>[6x]KNKLYKNIEIDTDTHSVYIHSENKKILLNLTL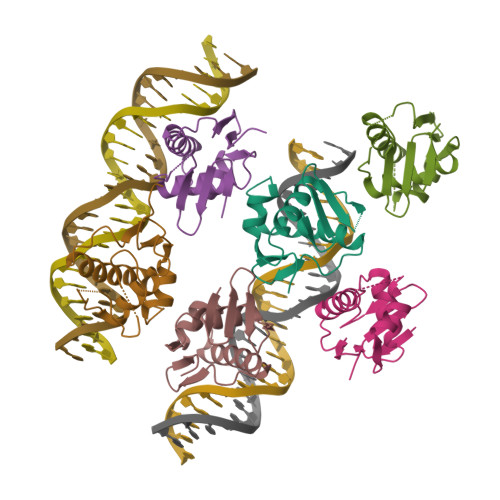TEYKIISFMIDQPHKVFTRGELMNHCMNDSDALERTVDSHVSKLRKKLEEQGIFQMLINVRGVGYRLDNPLAVKDDA2-[2-[(2-azanyl-4-oxidanylidene-1H-pteridin-7-yl)carbonylamino]ethanoylamino]ethanoic 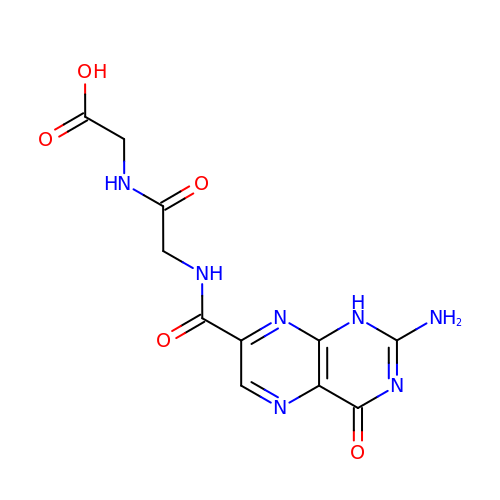acid | C11 H11 N7 O5 | WMBGGQNJJUXOQV-UHFFFAOYSA-N>MGSSHHHHHHSSGRENLYFQGHVTSDPGTAAPVKRTAEQSRSLIVDAAGRAFATRPYREITLKDIAEDAGVSAPLIIKYFGSKEQLFDALVDFRAAAEIVFSGPLDGLGERMVSMFARPLEPYKPLSLNILFMSGPSEESSRKLRANYSAQMIDALAERLPGRDARLRAELVMSMLTGLAVMRRKMMQEHATGTPEEVVAHYAPLVQELLDGGS[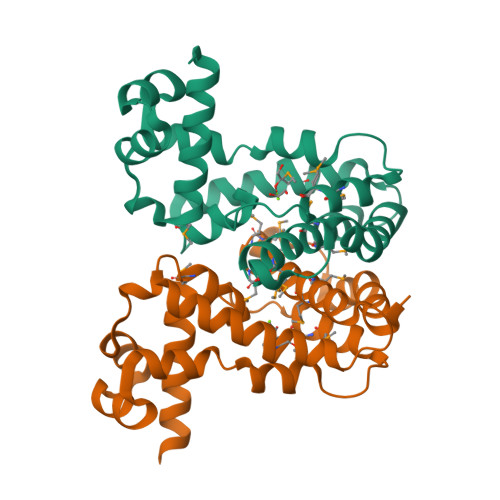2x]> RATPV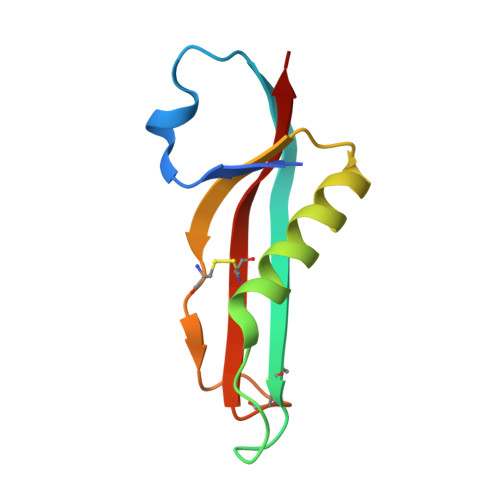RIYTNAEELVGKPFRDLGEVSGDSCQASNQDSPPSIPTARKRMQINASKMKANAVLLHSCEVTSGTPGCYRQAVCIGSALNIT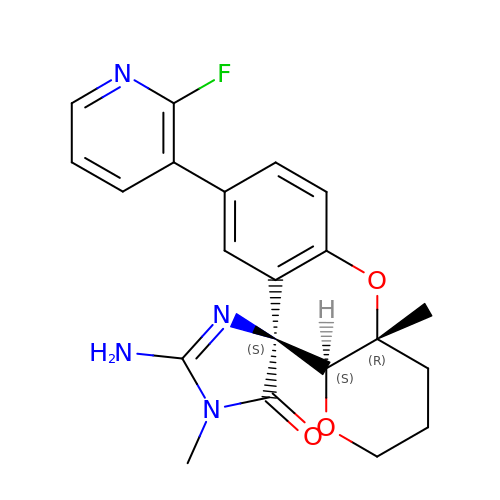(4S,4a'R,10a'S)-2-amino-8'-(2-fluoropyridin-3-yl)-1,4a'-dimethyl-3',4',4a',10a'-tetrahydro-2'H-spiro[imidazole-4,10'-pyrano[3,2-b]chromen]-5(1H)-one | C21 H21 F N4 O3 | RYCBSDWTFORSET-UIFIKXQLSA-N> KEYTLDKAHTDVGFKIKHLQISNVKGNFKDYSAVI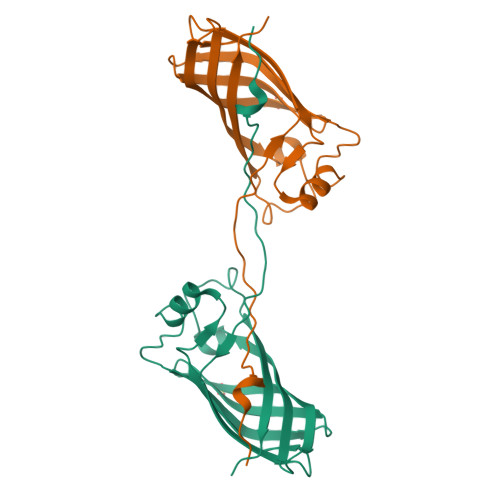DFDPASAEFKKLDVTIKIASVNTENQTRDNHLQQDDFFKAKKYPDMTFTMKKYEKIDNEKGKMTGTLTIAGVSKDIVLDAEIGGVAKGKDGKEKIGFSLNGKIKRSDFKFATSTSTITLSDDINLNIEVEANEKEGGSHHHHHH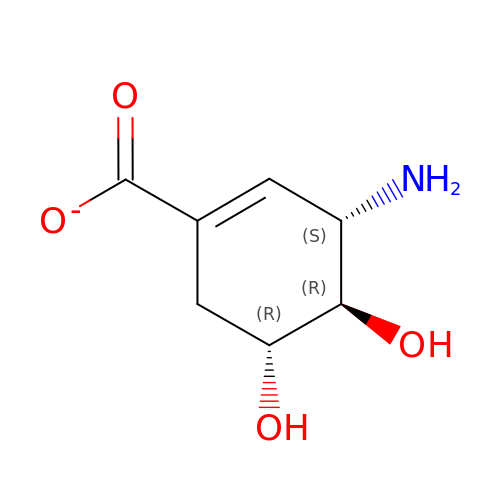3-AMINO-4,5-DIHYDROXY-CYCLOHEX-1-ENECARBOXYLATE | C7 H10 N O4 | WPZSUTUAATWRPU-KVQBGUIXSA-M2-{[(2R)-2-HYDROXY-3-(9-PHENANTHRYLOXY)PROPYL]AMINO}PROPANE-1,3-DIOL 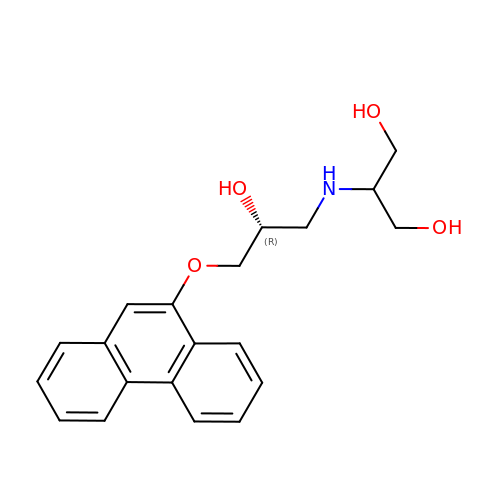| C20 H23 N O4 | WXMOCMHFWHZBSU-MRXNPFEDSA-N> MAARLLAPPGPDSFKPFTPESLANIERRIAESKLKKPPKADGSHREDDEDSKPKPNSDLEAGKSLPFIYGDIPQGLVAVPLEDFDPYYLTQKTFVVLNRGKTLFRFSATPALYILSPFNLIRRIAIKILIHSVFSMIIMCTILTNCVFMTFSNPPDWSKNVEYTFTGIYTFESLVKIIARGFCIDGFTFLRDPWNWLDFSVIMMAYITEFVNLGNVSALRTFRVLRALKTISVIPGLKTIVGALIQSVKKLSDVMILTVFCLSVFALIGLQLFMGNLRNKCVVWPINFNESYLENGTKGFDWEEYINNKTNFYTVPGMLEPLLCGNSSDAGQCPEGYQCMKAGRNPNYGYTSFDTFSWAFLALFRLMTQDYWENLYQLTLRAAGKTYMIFFVLVIFVGSFYLVNLILAVVAMAYEEQNQATLEEAEQKEAEFKAMLEQLKKQQEEAQAAAMATSAGTVSEDAIEEEGEEGGGSPRSSSEISKLSSKSAKERRNRRKKRKQKELSEGEEKGDPEKVFKSESEDGMRRKAFRLPDNRIGRKFSIMNQSLLSIPGSPFLSRHNSKSSIFSFRGPGRFRDPGSENEFADDEHSTVEESEGRRDSLFIPIRARERRSSYSGYSGYSQGSRSSRIFPSLRRSVKRNSTVDCNGVVSLIGGPGSHIGGRLLPEATTEVEIKKKGPGSLLVSMDQLASYGRKDRINSIMSVVTNTLVEELEESQRKCPPCWYKFANTFLIWECHPYWIKLKEIVNLIVMDPFVDLAITICIVLNTLFMAMEHHPMTPQFEHVLAVGNLVFTGIFTAEMFLKLIAMDPYYYFQEGWNIFDGFIVSLSLMELSLADVEGLSVLRSFRLLRVFKLAKSWPTLNMLIKIIGNSVGALGNLTLVLAIIVFIFAVVGMQLFGKSYKECVCKINQDCELPRWHMHDFFHSFLIVFRVLCGEWIETMWDCMEVAGQAMCLIVFMMVMVIGNLVVLNLFLALLLSSFSADNLAATDDDGEMNNLQISVIRIKKGVAWTKLKVHAFMQAHFKQREADEVKPLDELYEKKANCIANHTGADIHRNGDFQKNGNGTTSGIGSSVEKYIIDEDHMSFINNPNLTVRVPIAVGESDFENLNTEDVSSESDPEGSKDKLDDTSSSEGSTIDIKPEVEEVPVEQPEEYLDPDACFTEGCVQRFKCCQVNIEEGLGKSWWILRKTCFLIVEHNWFETFIIFMILLSSGALAFEDIYIEQRKTIRTILEYADKVFTYIFILEMLLKWTAYGFVKFFTNAWCWLDFLIVAVSLVSLIANALGYSELGAIKSLRTLRALRPLRALSRFEGMRVVVNALVGAIPSIMNVLLVCLIFWLIFSIMGVNLFAGKYHYCFNETSEIRFEIEDVNNKTECEKLMEGNNTEIRWKNVKINFDNVGAGYLALLQVATFKGWMDIMYAAVDSRKPDEQPKYEDNIYMYIYFVIFIIFGSFFTLNLFIGVIIDNFNQQKKKFGGQDIFMTEEQKKYYNAMKKLGSKKPQKPIPRPLNKIQGIVFDFVTQQAFDIVIMMLICLNMVTMMVETDTQSKQMENILYWINLVFVIFFTCECVLKMFALRHYYFTIGWNIFDFVVVILSIVGMFLADIIEKYFVSPTLFRVIRLARIGRILRLIKGAKGIRTLLFALMMSLPALFNIGLLLFLVMFIFSIFGMSNFAYVKHEAGIDDMFNFETFGNSMICLFQITTSAGWDGLLLPILNRPPDCSLDKEHPGSGFKGDCGNPSVGIFFFVSYIIISFLIVVNMYIAIILENFSVATEESADPLSEDDFETFYEIWEKFDPDATQFIEYCKLADFADALEHPLRVPKPNTIELIAMDLPMVSGDRIHCLDILFAFTKRVLGDSGELDILRQQMEERFVASNPSKVSYEPITTTLRRKQEEVSAVVLQRAYRGHLARRGFICKKTTSNKLENGGTHREKKESTPSTASLPSYDSVTKPEKEKQQRAEEGRRERAKRQKEVRESKC;> MHRDAWLPRPAFSLTGLSLFFSLVPPGRSMEVTVPATLNVLNGSDARLPCTFNSCYTVNHKQFSLNWTYQECNNCSEEMFLQFRMKIINLKLERFQDRVEFSGNPSKYDVSVMLRNVQPEDEGIYNCYIMNPPDRHRGHGKIHLQVLMEEPPERDSTVAVIVGASVGGFLAVVILVLMVVKCVRRKKEQKLSTDDLKTEEEGKTDGEGNPDDGAK;> MGRLLALVVGAALVSSACGGCVEVDSETEAVYGMTFKILC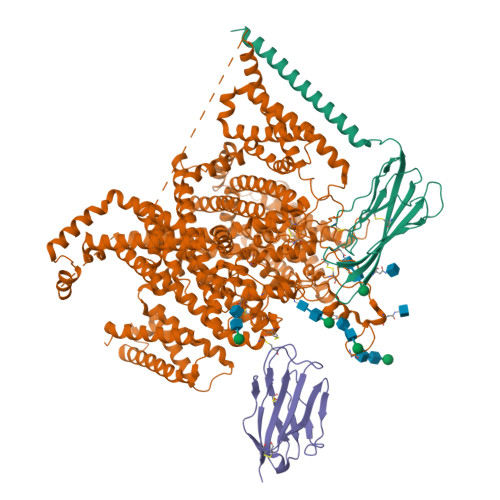ISCKRRSETNAETFTEWTFRQKGTEEFVKILRYENEVLQLEEDERFEGRVVWNGSRGTKDLQDLSIFITNVTYNHSGDYECHVYRLLFFENYEHNTSVVKKIHIEVVDKANRDMASIVSEIMMYVLIVVLTIWLVAEMIYCYKKIAAATETAAQENASEYLAITSESKENCTGVQVAE> MLKRKQSSRVEAQPVTDFGPDESLSDNADILWINKPWVHSLLRICAIISVISVCMNTPMTFEHYPPLQYVTFTLDTLLMFLYTAEMIAKMH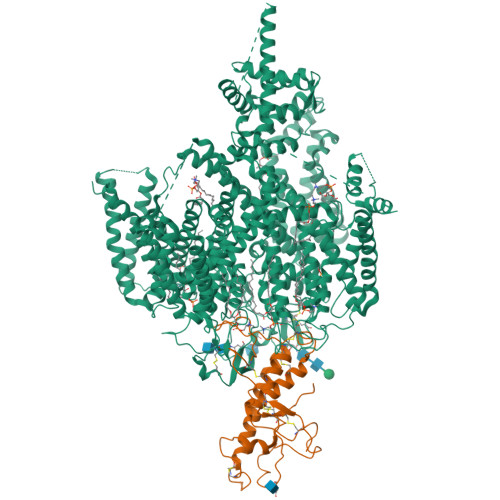IRGIVKGDSSYVKDRWCVFDGFMVFCLWVSLVLQVFEIADIVDQMSPWGMLRIPRPLIMIRAFRIYFRFELPRTRITNILKRSGEQIWSVSIFLLFFLLLYGILGVQMFGTFTYHCVVNDTKPGNVTWNSLAIPDTHCSPELEEGYQCPPGFKCMDLEDLGLSRQELGYSGFNEIGTSIFTVYEAASQEGWVFLMYRAIDSFPRWRSYFYFITLIFFLAWLVKNVFIAVIIETFAEIRVQFQQMWGSRSSTTSTATTQMFHEDAAGGWQLVAVDVNKPQGRAPACLQKMMRSSVFHMFILSMVTVDVIVAASNYYKGENFRRQYDEFYLAEVAFTVLFDLEALLKIWCLGFTGYISSSLHKFELLLVIGTTLHVYPDLYHSQFTYFQVLRVVRLIKISPALEDFVYKIFGPGKKLGSLVVFTASLLIVMSAISLQMFCFVEELDRFTTFPRAFMSMFQILTQEGWVDVMDQTLNAVGHMWAPVVAIYFILYHLFATLILLSLFVAVILDNLELDEDLKKLKQLKQSEANADTKEKLPLRLRIFEKFPNRPQMVKISKLPSDFTVPKIRESFMKQFIDRQQQDTCCLLRSLPTTSSSSCDHSKRSAIEDNKYIDQKLRKSVFSIRARNLLEKETAVTKILRACTRQRMLSGSFEGQPAKERSILSVQHHIRQERRSLRHGSNSQRISRGKSLETLTQDHSNTVRYRNAQREDSEIKMIQEKKEQAEMKRKVQEEELRENHPYFDKPLFIVGREHRFRNFCRVVVRARFNASKTDPVTGAVKNTKYHQLYDLLGLVTYLDWVMIIVTICSCISMMFESPFRRVMHAPTLQIAEYVFVIFMSIELNLKIMADGLFFTPTAVIRDFGGVMDIFIYLVSLIFLCWMPQNVPAESGAQLLMVLRCLRPLRIFKLVPQMRKVVRELFSGFKEIFLVSILLLTLMLVFASFGVQLFAGKLAKCNDPNIIRREDCNGIFRINVSVSKNLNLKLRPGEKKPGFWVPRVWANPRNFNFDNVGNAMLALFEVLSLKGWVEVRDVIIHRVGPIHGIYIHVFVFLGCMIGLTLFVGVVIANFNENKGTALLTVDQRRWEDLKSRLKIAQPLHLPPRPDNDGFRAKMYDITQHPFFKRTIALLVLAQSVLLSVKWDVEDPVTVPLATMSVVFTFIFVLEVTMKIIAMSPAGFWQSRRNRYDLLVTSLGVVWVVLHFALLNAYTYMMGACVIVFRFFSICGKHVTLKMLLLTVVVSMYKSFFIIVGMFLLLLCYAFAGVVLFGTVKYGENINRHANFSSAGKAITVLFRIVTGEDWNKIMHDCMVQPPFCTPDEFTYWATDCGNYAGALMYFCSFYVIIAYIMLNLLVAIIVENFSLFYSTEEDQLLSYNDLRHFQIIWNMVDDKREGVIPTFRVKFLLRLLRGRLEVDLDKDKLLFKHMCYEMERLHNGGDVTFHDVLSMLSYRSVDIRKSLQLEELLAREQLEYTIEEEVAKQTIRMWLKKCLKRIRAKQQQSCSIIHSLRESQQQELSRFLNPPSIETTQPSEDTNANSQDNSMQPETSSQQQLLSPTLSDRGGSRQDAADAGKPQRKFGQWRLPSAPKPISHSVSSVNLRFGGRTTMKSVVCKMNPMTDAASCGSEVKKWWTRQLTVESDESGDDLLDILEDEVDAGSDYKDDDDKGSDYKDDDDK;> MTRGAWMCRQYDDGLKIWLAAPRENEKPFIDSERAQKWRLSLASLLFFTVLLSDHLWFCAEAKLTRARDKEHQQQQRQQQQQQQQQRQRQQQQQQRRQQEPSWPALLASMGESSPAAQAHRLLSASSSPTLPPSPGDGGGGGGKGNRGKDDRGKALFLGNSAKPVWRLETCYPQGASSGQCFTVENADAVCARNWSRGAAGGDGQEVRSKHPTPLWNLSDFYLSFCNSYTLWELFSGLSSPNTLNCSLDVVLKEGGEMTTCRQCVEAYQDYDHHAQEKYEEFESVLHKYLQSEEYSVKSCPEDCKIVYKAWLCSQYFEVTQFNCRKTIPCKQYCLEVQTRCPFILPDNDEVIYGGLSSFICTGLYETFLTNDEPECCDVRREEKSNNPSKGTVEKSGSCHRTSLTVSSATRLCNSRLKLCVLVLILLHTVLTASAAQNTAGLSFGGINTLEENSTNEELEDEVDAGSDYKDDDDKGSDYKDDDDK> MTPSPEASEGPCVSKLRNEPLGALTPYVGVVDGPEVKKSKKIHGGDSAILGTYKMQSRFNRGVLLMVNIMDYPDQNRRRIGAEKDSKSLIHLFQELNFTIFPYGNVNQDQFFKLLTMVTSSSYVQNTECFVMVLMTHGNSVEGKEKVEFRDGSVVDMQKIKDHFQTAKCPYLVNKPKVLMFPFARGDEYDLGHPKNQGNLMEPVY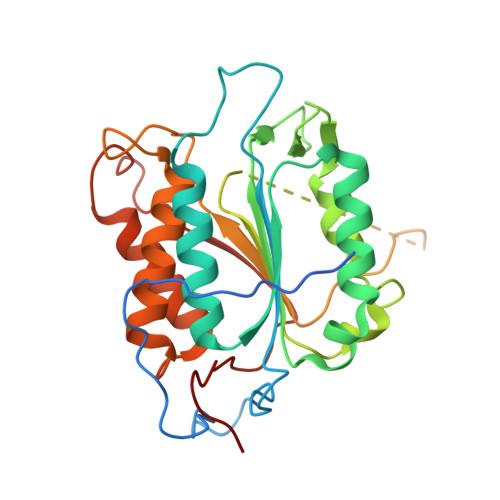TAQEEKWPDTQTEGIPSPSTNVPSLADTLVCYANTPGYVTHRDLDTGSWYIQKFCQVMADHAHDTDLEDILKKTSEAVGNKRTKKGSMQTGAYDNLGFNKKLYFNPGFFNE> MEDIIVVALYDYVSWSPDDLSFQKGDQMVVLEESGEWWK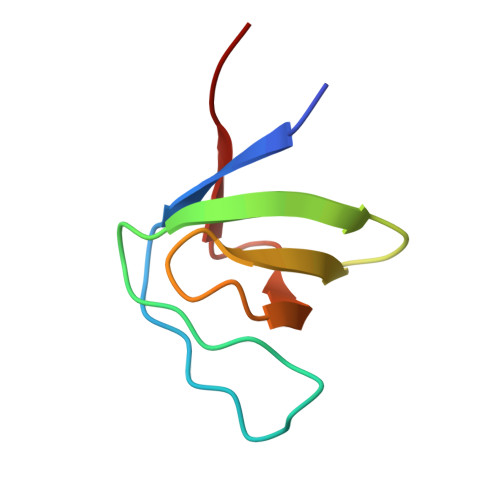ARSLATRKEGYIPSNYVARVDS> SPNIEACGYSDRVLQLTLGNSTITTQEAANSVVAYGRWPEYLRDSEANPVDQPTEPDVAACRFYTLDTVSWTKESRGWWWKLPDALRDMGLFGQNMYYHYLGRSGYTVHVQCNASKFHQGALGVFAVPEMCLAGDSNTTTMYTSYQNANPGEKGGTFTGTFTPDNNQTSPARRFCPVDYLLGNGTLLGNAFVFPHQI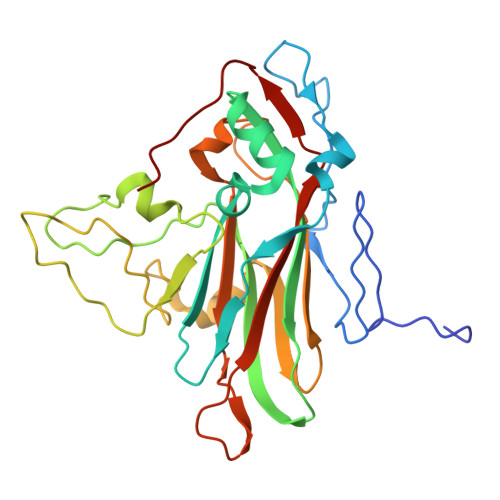INLRTNNCATLVLPYVNSLSIDSMVKHNNWGIAILPLAPLNFASESSPEIPITLTIAPMCCEFNGLRNITLPRLQ(3S,6S)-3-((R)-2,3-dihydroxy-2-methylpropyl)-6-((S)-4-hydroxybutan-2-yl)piperazine-2,5-dione 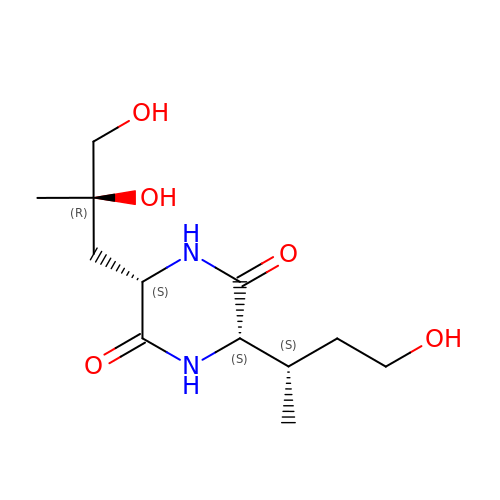| C12 H22 N2 O5 | YLDBCWRFRZSTCF-PHGLEFOZSA-N>[4x]MSYTVGTYLAERLVQIGLKHHFAVAGDYNLVLLDNLLLNKNMEQVYCCNELNCGFSAEGYARAKGAAAAVVTYSVGALSAFDAIGGAYAENLPVILISGAPNNNDHAAGHVLHHALGKTDYHYQLEMAKNITAAAEAIYTPEEAPAKIDHVIKTALREKKPVYLEIACNIASMPCAAPGPASALFNDEASDEASLNAAVEETLKFIANRDKVAVLVGSKLRAAGAEEAAVKFADALGGAVATMAAAKSFFPEENPHYIGTSWGEVSYPGVEKTMKEADAVIALAPVFNDYSTTGWTDIPDPKKLVLAEPRSVVVNGIRFPSVHLKDYLTRLAQKVSKKTGALDFFKSLNAGELKKAAPADPSAPLVNAEIARQVEALLTPNTTVIAETGDSWFNAQRMKLPNGARVEYEMQWGHIGWSVPAAFGYAVGAPERRNILMVGDGSFQLTAQEVAQMVRLKLPVIIFLINNYGYTIAVMIHDGPYN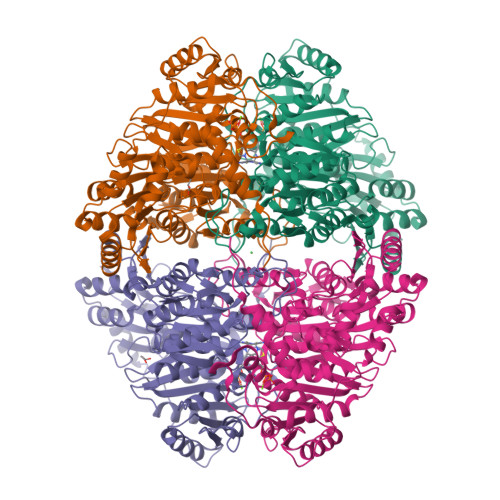NIKNWDYAGLMEVFNGNGGYDSGAGKGLKAKTGGELAEAIKVALANTDGPTLIECFIGREDCTEELVKWGKRVAAANSRKPVNKLL>[4x]MSRVAIVTGASSGNGLAIATRFLARGDRVAALDLSAETLEETARTHWHAYADKVLRVRADVADEGDVNAAIAATMEQFGAIDVLVNNAG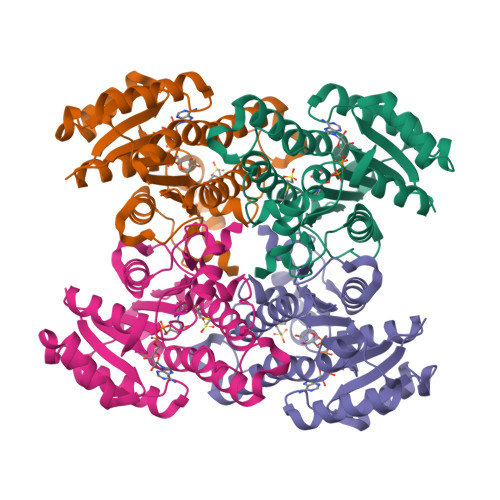ITGNSEAGVLHTTPVEQFDKVMAVNVRGIFLGCRAVLPHMLLQGAGVIVNIASVASLVAFPGRSAYTTSKGAVLQLTKSVAVDYAGSGIRCNAVCPGMIETPMTQWRLDQPELRDQVLARIPQKEIGTAAQVADAVMFLAGEDATYVNGAALVMDGAYTAI> ASMKQPVVVIGSGLAGLTTSNRLISKYRIPVVLLDKAASIGGNSIKASSGINGAHTDTQQNLKVMDTPELFLKDTLHSAKGRGVPSLMDKLTKESKSAIRWLQTEFDLKLDLLAQLGGHSVPRTHRSSGKLPPGFEIVQALSKKLKDISSKDSNLVQIMLNSEVVDIELDNQGHVTGVVYMDENGNRKIMKSHHVVFCSGGFGYSKEMLKEYSPNLIHLPTTNGKQTTGDGQKILSKLGAELIDMDQVQVHPTGFIDPNDRENNWKFLAAEALRGLGGILLHPTTGRRFTNELSTRDTVTMEIQSKCPKNDNRALLVMSD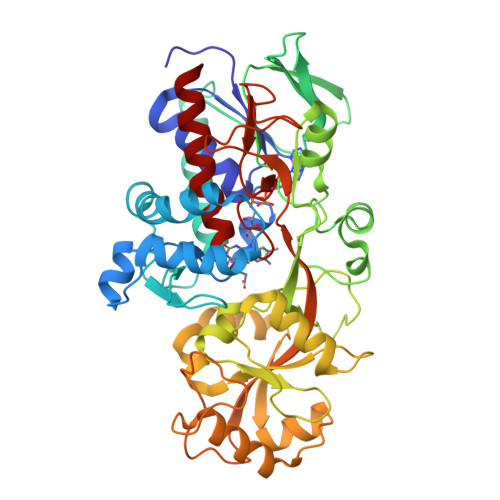KVYENYTNNINFYMSKNLIKKVSINDLIRQYDLQTTASELVTELKSYSDVNTKDTFDRPLIINAFDKDISTESTVYVGEVTPVVHFTMGGVKINEKSQVIKKNSESVLSNGIFAAGEVSGGVHGANRLGGSSLLECVVFGKTAADNIAKLY>GNSDGQLDTHLADLYLLKYDTGLGVYESFICKYLEDSNDYIASHPQKLSLDE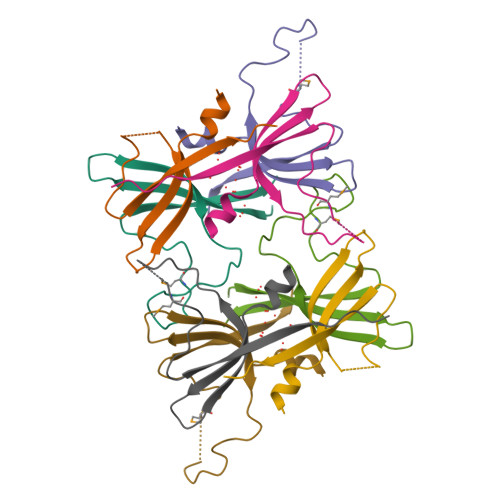MPRPLESETVSLRQLIVSVLPSRPSI[4x]>TQQNTPLADDTTLMSTTDLQGYITHANDTFVQVSGYTLQELQGQPHNMVRHPDMPKAVFADMWFTLKKGEPWSGIVKNRRKNGDHYWVRANVVPMVREGKISGYMSIRTRATDEEIAAVEPLYKALN[2x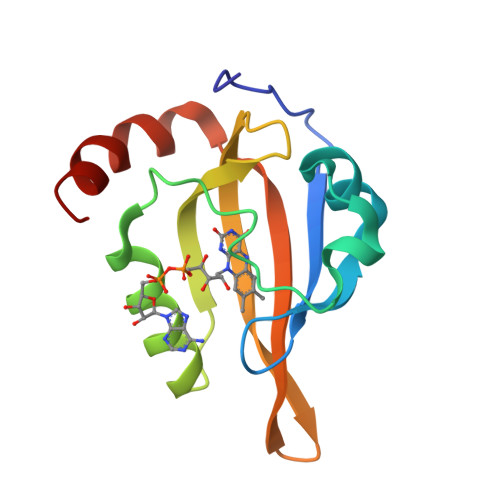]> GPLGSMVSGVGGSGGGRGGGRGGEEEPSSSHTPNNRRGGEQAQSSGTKSLRPRSNTESMSKAIQQYTVDARLHAVFEQSGESGKSFDYSQSLKTTTYGSSVPEQQITAYLSRIQRGGYIQPFGCMIAVDESSFRIIGYSENAREMLGIMPQSVPTLEKPEILAMGTDVRSLFTSSSSILLERAFVAREITLLNPVWIHSKNTGKPFYAILHRIDVGVVIDLEPARTEDPALSIAGAVQSQKLAVRAISQLQALPGGDIKLLCDTVVESVRDLTGYDRVMVYKFHEDEHGEVVAESKRDDLEPYIGLHYPATDIPQASRFLFKQNRVRMIVDCNATPVLVVQDDRLTQSMCLVGSTLRAPHGCHSQYMANMGSIASLAMAVIINGNEDDGSNVASGRSSMRLWGLVVCHHTSSRCIPFPLRYACEFLMQAFGLQLNMELQLALQMSEKRVLRTQTLLCDMLLRDSPAGIVTQSPSIMDLVKCDGAAFLYHGKYYPLGVAPSEVQIKDVVEWLLANHADSTGLSTDSLGDAGYPGAAALGDAVCGMAVAYITKRDFLFWFRSHTAKEIKWGGAKHHPEDKDDGQRMHPRSSFQAFLEVVKSRSQPWETAEMDAIHSLQLILRDSFKESEAAMNSKVVDGVVQPCRDMAGE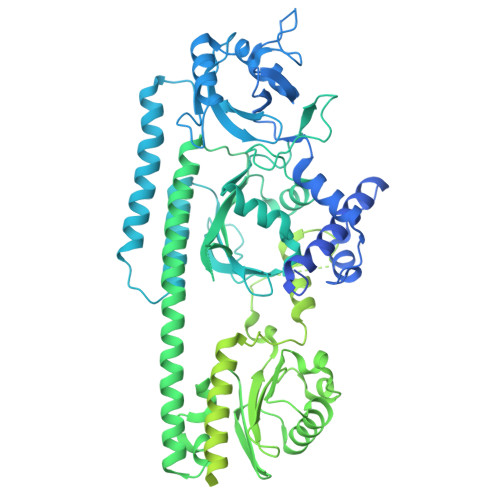QGIDELGAVAREMVRLIETATVPIFAVDAGGCINGWNAKIAELTGLSVEEAMGKSLVSDLIYKENEATVNKLLSRALRGDEEKNVEVKLKTFSPELQGKAVFVVVNACSSKDYLNNIVGVCFVGQDVTSQKIVMDKFINIQGDYKAIVHSPNPLIPPIFAADENTCCLEWNMAMEKLTGWSRSEVIGKMIVGEVFGSCCMLKGPDALTKFMIVLHNAIGGQDTDKFPFPFFDRNGKFVQALLTANKRVSLEGKVIGAFCFLQIPSPELQQALAVQRRQDTECFTKAKELAYICQVIKNPLSGMRFANSLLEATDLNEDQKQLLETSVSCEKQISRIVGDMDLESIEDGSFVLKREEFFLGSVINAIVSQAMFLLRDRGLQLIRDIPEEIKSIEVFGDQIRIQQLLAEFLLSIIRYAPSQEWVEIHLSQLSKQMADGFAAIRTEFRMACPGEGLPPELVRDMFHSSRWTSPEGLGLSVCRKILKLMNGEVQYIRESERSYFLIILELPVPRKRPLSTASGSGDMMLMMPY>[2x]MGHHHHHHENLYFQGVQKIGILGAMREEITPILELFGVDFEEIPLGGNVFHKGVYHNK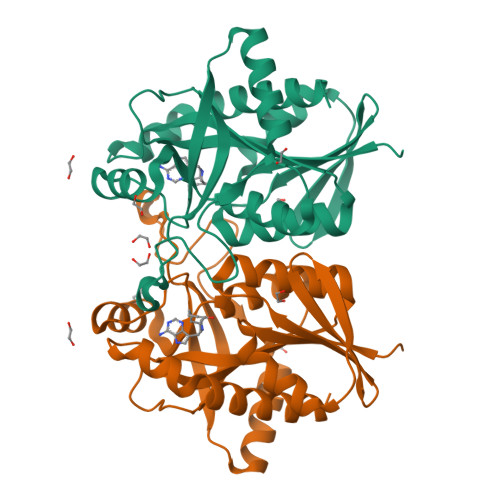EIIVAYSKIGKVHSTLTTTSMILAFGVQKVLFSGVAGSLVKDLKINDLLVATQLVQHDVDLSAFDHPLGFIPESAIFIETSGSLNALAKKIANEQHIALKEGVIASGDQFVHSKERKEFLVSEFKASAVEMEGASVAFVCQKFGVPCCVLRSISDNADEKAGMSFDEFLEKSAHTSAKFLKSMVDEL>[2x]HPETLVKVKDAEDQLGARVGYIELDLNSGKILESFRPEERFPMMSTFKVLLCGAVLSRIDAGQEQLGRRIHYSQNDLVYNSPVTEKHLTDGMTVRELCSAAITMSDNTAANLLLTTIGGPKELTAFLHNMGDHVTRLDRWEPELNEAIPNDERDTTMPAAMATTLRKLLTGELLTLASRQQLIDWMEADKVAGPLLRSALPA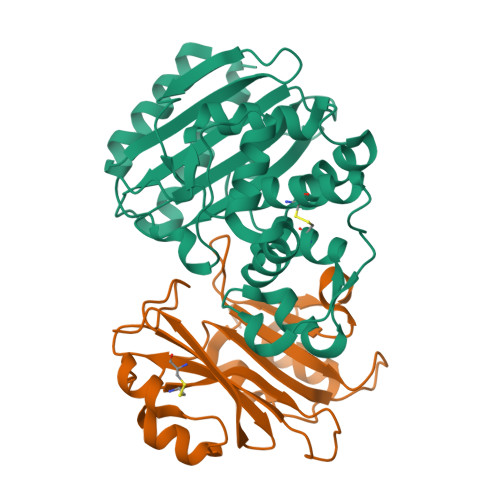GWFIADKSGAGERGSRGIIAALGPDGKPSRIVVIYTTGSQATMDERNRQIAEIGASLIKHW;>AGVMTGAKFTQIQFGMTRQQVLDIAGAENCETGGSFGDSIHCRGHAAGDYYAYATFGFTSAAADAKVDSKSQEKLLAPSAPTLTLAKFNQVTVGMTRAQVLATVGQGSCTTWSEYYPAYPSTAGVTLSLSCFDVDGYSSTGFYRGSAHLWFTDGVLQGKRQWDLV[2x]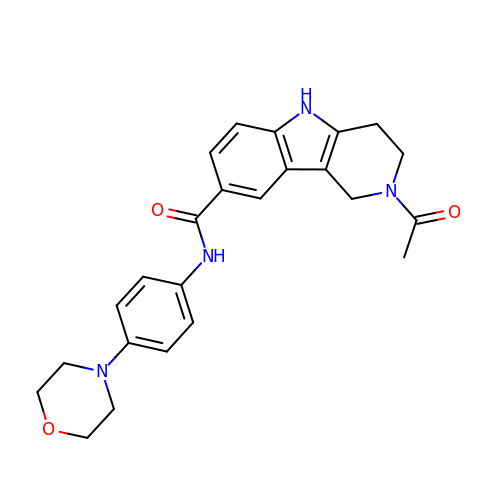2-ethanoyl-~{N}-(4-morpholin-4-ylphenyl)-1,3,4,5-tetrahydropyrido[4,3-b]indole-8-carboxamide | C24 H26 N4 O3 | SWCZIQFQNPAUEC-UHFFFAOYSA-N> MAPVPEPEVVATPPADAGRGLIRVDSREIRHYSGTRKEPDYLVSRDNGKTWEMKAAPAGYPPNYGGIPKESPAIVRNPLTREFIRVQPIGGFVFLSRGGLDGKWLAVTNDGKLEEDWKDPEKRKNLKKLGGIMRTPVFVNKGRRVIVPFHNMGGGTKFHISDDGGLTWHVSRNGVTSPRHEARPPHQGVRWFNNAVEATVLEMKDGTLWALARTSQDQAWQAFSKDYGETWSKPEPSRFFGTLTMNTLGRLDDGTIVSLWTNTMALPENATAGNGTWEDVFTNRDSHHIAMSGDEGKTWYGFREIILDEHRNHPGYATLDGPEDRGKHQSEMVQLDKNRILISLGQHKNHRRLVIVDRRWVGAKTRATQTGKDLDSQWTIHTYIPQKKGHCSYNRKPSA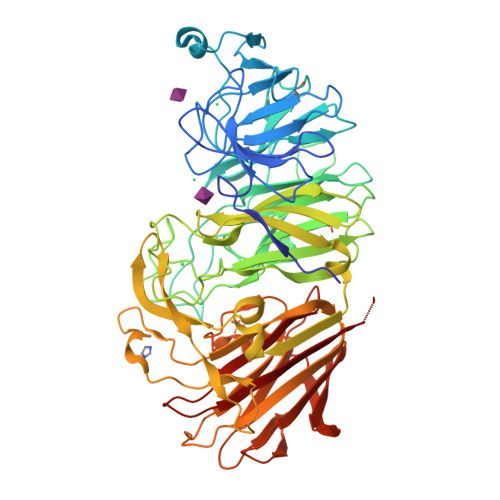ELVQDPSGGTKKVLQIKRLDDPELVNEKSNVDYRNGGATWNFPNGTTGLVKFRFRVVDGEQADDSGLQVSLTDRLFNACDSTTKDYALFTFPIRLKPAPHLLLGMKKVPFTPGAWHEISLLWQGGQAVVSLDGKKAGTLKMANKSPNGASYIHFISTGSQPDAGILLDTVNARVKAAAA;> MAPVPEPEVVATPPADAGRGLIRVDSREIRHYSGTRKEPDYLVSRDNGKTWEMKAAPAGYPPNYGGIPKESPAIVRNPLTREFIRVQPIGGFVFLSRGGLDGKWLAVTNDGKLEEDWKDPEKRKNLKKLGGIMRTPVFVNKGRRVIVPFHNMGGGTKFHISDDGGLTWHVSRNGVTSPRHEARPPHQGVRWFNNAVEATVLEMKDGTLWALARTSQDQAWQAFSKDYGETWSKPEPSRFFGTLTMNTLGRLDDGTIVSLWTNTMALPENATAGNGTWEDVFTNRDSHHIAMSGDEGKTWYGFREIILDEHRNHPGYATLDGPEDRGKHQSEMVQLDKNRILISLGQHKNHRRLVIVDRRWVGAKTRATQTGKDLDSQWTIHTYIPQKKGHCSYNRKPSAELVQDPSGGTKKVLQIKRLDDPELVNEKSNVDYRNGGATWNFPNGTTGLVKFRFRVVDGEQADDSGLQVSLTDRLFNACDSTTKDYALFTFPIRLKPAPHLLLGMKKVPFTPGAWHEISLLWQGGQAVVSLDGKKAGTLKMANKSPNGASYIHFISTGSQPDAGILLDTVNARVKAE> MNVKEMDFNDLSNKSNQIINRISSFSSPIGLSSFNIERNLQEIGDTSKQLNDLTSSKTPFSNPLEPNVFQDSKINRKYGLDPKVLAKNLSNINTSSFTDVQSVPTDIDGYLKVQFENIILNTICDIQKKTSKEFQSHYEQTSIHDWNRDKKYLEEILGQKHIKVLPSVGGASASNQSSSSSSLFQQSVRGGLSSSIMGQSVRPTYGQQSQFGGSSTISIGGNISRVGGGSGGGIYSQRQTGQNEDRTKLSDKMKKYASIIEEYDIHMADQSKSYGFPLVHRLMDACLSTDINIGGGINTNTATTIVTHVWNLLLTLTSEIDTTNYIQQLKEQQQQQQQQTPQLKEQQQKQQQLTELQKHTKYHTKPTMAQLLKRSISFLETQFSQVIESRLPKHSNVSLPLNIIVAYIKSLNQSPLTDSSDEIYEGCSIWCIIYYLLRSGYTLEAYQFALEKCGSRYFDILSPIFKEKQQQQQQQQQQQQQQQQQQQQKSSLPTTTNNTSINKDQRDRMTREFNTAKTESKDVFKISVFNLLSCNDPNSTKQQ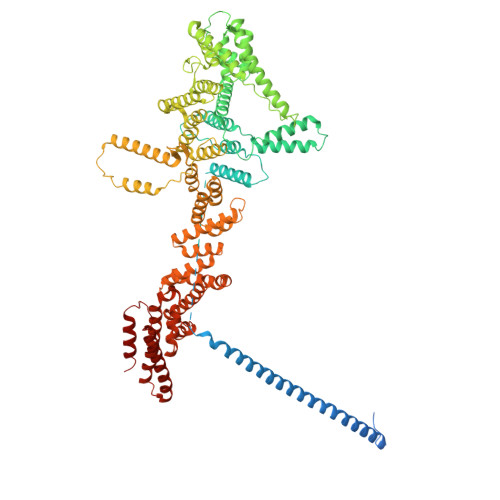VITSIQDYIWWRLNFIRERITIEPTNDSAISLLESLQNDIKNSIEKNRNNYETLEIFQLLLVSLQFEDAIVSLYQFCPDDSLHLAIALDYYKLLRTSNSGINNKHVDEINKFNKSTTNTNTMTYQQNQQQQQQQQQQQQQEQQKEIYDQTSKSIHLVEMIKQYTKIFSFEENREAFFYYLLIADNDIKIQEISELVVSSPNGFKFAHELSLFSEFINKQQWRTIIEQSALELENKNEYQSAIEFWIMIEEYPRVLEIYNSRISVLLTSISSERDQLYQFGKQLFNDYQGRLKTTSTARTSYLAFEQLLKLCDFFDLYNKEKYQEAIQKIENLEILPISESEIDSKVQDYRFLSPHITRNFSSIIQAYVDIIVKQYHLLNNFDEFTNRSALFAGRKQTIQDLQSRTQCIALFAGKIDFPMSGNILPRLMNLFISMSN> GNSEEDYPNGTWLGDENNPEMRVRCAIIPSDMLHISTNCRTAEKMALTLLDYLFHREVQAVSNLSGQGKHGKKQLDPLTIYGIRCHLFYKFGITESDWYRIKQSIDSKCRTAWRRKQRGQSL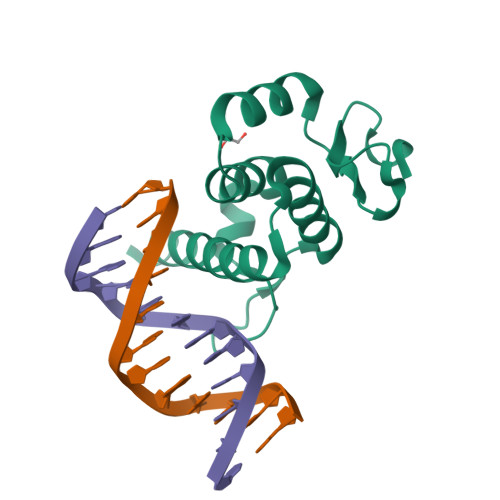AVKSFSRRTPNSSSYCPSE>MLMEAALPGSDVSAREVAKVWPGAKKGDYSFLQGNQSRSLEAEMTRTARAEAGTDRHRALKDYAVDADNLPKTLSAGSKHLTEDGDVIEARLDDAIPRMLFAASDPEYVDTLFREQLLEVVMEGRELRKVAREASNVINANTRVGDVPIASDEEFARPTGQGAEIRDDGETYTTVAWNATKLTEGSRVTDEMRDQAMVDLIERNIQRVGASLENGINRVFLTELVDNAQNNHDTAGSNQGYQALNSAVGEVDKDDFRPDTYVTHPDYRTQLFNDTNLAYANRAGTNEVLRNREDAPIVGDIAGLDMHAAMSSATYDDGTDIGWSGGSETWGFSSDGDKGAVVYDRDNIHTILYAPNGQDVEIKDYEDPIRDITGVNGRLHVDCQYSQGRSSATVQY[6x];>MTGLNPDGLGRTAAFSNTSAESVSAVDATIDRLYAQDRIEIPTDSRQLFSTRGTVLRNFEDLSGWTANIGSLSAETSDVYVGSQSARLTASSSAVDIRYSFGTAQDFTGKGFSMALKRIDVSGSSDSTPIKIRLVDGNTNYRTFSARCRPGGGDEWGRRDFGFESEDTGFDVTNVQTMTVTTNSRSSIDILVDDIRVVDSSGTGQVIVTIDDVHTGDKTAAEVFGRYGIPIGLAANAKFLDQSSSKLTTQEFKDLLAKPHVYAVNHGYNHYDYGSYSIDEIEDDVIRGKYELQDLGVREPNINHYVYPSGNYAQESIDMLSNYHVMSWGTGAESFDALTPNQLTSPWHNLRCSFDSGTAEAEQAVNDAATYNQTAHIYFHSDNVTQSEMESVAQTINSADVTPITLMDFYNQQ[3x];>MTDTIVNVQGSFFSASASGVADTESLLIDPQDAKFGAIEIHNIAHGGSVDVELLTSSDDTELVEDAAVTLDSFTGEGISQGNQIEASDNTNTYIRITNTSGGAIDIIATGREVSQ[6x]

Here, we present the near-atomic resolution structure of Haloferax tailed virus 1 (HFTV1), an archaeal virus thriving in extreme salinity. Through single-particle analysis, we obtained near-atomic resolution maps of DNA-filled and empty virions, enabling us to assemble full atomic models of the virus pre- and post-DNA release, including all structural protein components. The full atomic structure revealed that the virus has a length of 1350 Å and an icosahedral head with a diameter of ~600 Å. The tail has a length of 560 Å and terminates into a baseplate with three radiating TFs of ~190 Å in length.

Each hexagonal MCP of HFTV1 forms the base of a turret. The TBP inserts into the MCP hexamer with a short stalk formed by a six-stranded β-barrel. In icosahedral and asymmetric reconstructions of the capsid, the turret heads were poorly resolved, an indication of flexibility. To improve the resolution of the turret map, localized reconstruction techniques were used (flowchart S1). Particles were symmetry-expanded around the fivefold-symmetric head-tail axis, sampling the five particularly well-defined turret complexes adjacent to the portal. We found that the turrets are assembled in two possible orientations, where the turret head trimer can be rotated by 60° with respect to the turret base hexamer. This rotational flexibility may increase the chance of binding between turrets and the S-layer of H. gibbonsii. (E) Diagonal view of MCP5, showing that each MCP6 carries a turret, while all MCP5 remain unoccupied.> GPAMPPILDVIVIGGGQAALTTAYFLRRTSLSYLLLDEQPGPGGAWLHAWDSLRLFSPAAWSSIAGWPMPSPTEPGNPTRNDVIDYLRRYEDRYQFPIQRPVRVDTVTRLDDLWRVQAGDQQWLARAVISATGTWSKPFIPPYEGRELFQGAQIHSAHYRTPAPFAGKRVMVVGGGNSGAQVLAELSSVSETLWITQEPPAFLPDEVDGRVLFERATARWKAQQEGRSIDEPAGGFGDIVMVPPVREARERGVLVAERPFARFTETGVEWADGRREN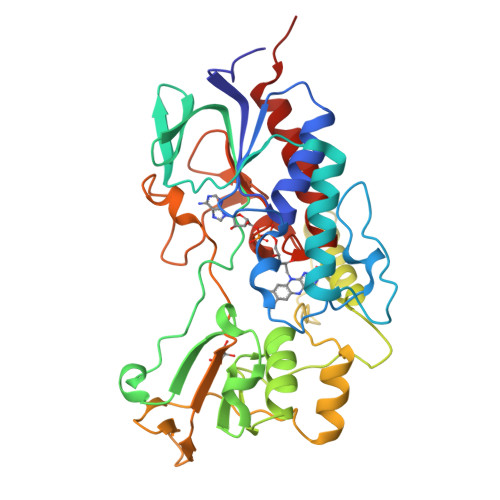LDAVIWCSGFRPALDHLRELGVVEADGKVQVEDTRVVKQPNLWLVGYGDWTGMASATLIGVTRTARSTADQVVQALTATPSRRP> R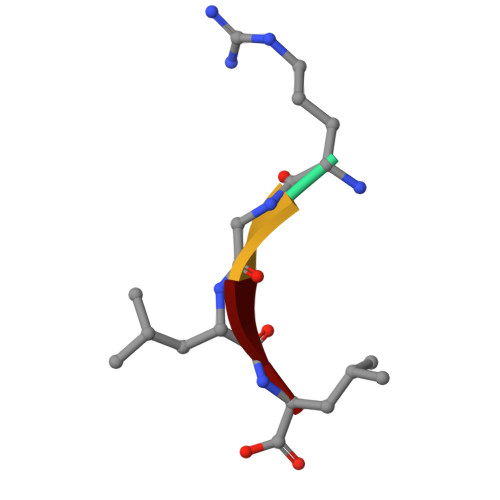GLL PfRh5 forms a complex with cysteine-rich protective antigen (CyRPA) and P. falciparum Rh5 interacting protein (PfRipr). The PfRh5/CyRPA/PfRipr complex plays an essential role for invasion of P. falciparum into human erythrocytes through binding the receptor basigin. CyRPA displays a canonical six-bladed β-propeller fold, and the inhibitory monoclonal is shown to block formation of the PfRh5/CyRPA complex. Within the β-propeller structure are four intra-sheet disulfide bonds (Cys19-Cys35, Cys90-Cys92, Cys151-Cys169 and Cys229-Cys239) and one inter-sheet disulfide bond (Cys274-Cys298).

To provide a structural basis for understanding the function of this complex and its components we have determined the structure of CyRPA in its free form. Crystals were also obtained of uncomplexed CyRPA; this structure was determined by molecular replacement, using the CyRPA component of the Fab-complexed structure as a search model, and subsequently refined using diffraction data to 3.09 Å resolution. The crystal of uncomplexed CyRPA contains four copies of the protein in the crystallographic asymmetric unit, arranged with approximate 222-point group symmetry. Within this tetramer, a pairwise association of CyRPA molecules is mediated by the formation of two eight-strand anti-parallel β-sheets, one (termed sheet ‘6–6’) comprises two copies of the sixth β-sheet of the CyRPA monomer and the second (termed sheet ‘5–5’) comprises two copies of the (adjacent) fifth β-sheet of the CyRPA monomer. In each case, formation of the eight-stranded sheet is mediated by the respective outermost strands of the two constituent four-stranded sheets. These dimers of CyRPA monomers then associate with each other via the formation of a β-sandwich comprising sheet 6–6 of one CyRPA dimer and sheet 6–6 of the second CyRPA dimer. The monomer-monomer interfaces, although extensive, are most likely an artefact of crystallization, as we find no evidence for higher-order association upon SEC of CyRPA. However, we cannot rule out such associations occurring within the hetero-complexes formed by CyRPA and its partner proteins on the surface of the merozoite. The closest structural homologue to CyRPA is the attachment glycoprotein of a henipah virus which binds to ephrinB2 and is important for host cell entry; however, it also has some similarity to bacterial and viral sialidases all of which have a six-bladed β-propeller fold. CyRPA lacks some of the important amino acid motifs required for it to be an active sialidase, and the recombinant form of the protein did not have sialidase activity suggesting it is only distantly related to these enzymes.

>[4x]GTSRHVFIRTELSFIKNNVPCIRDMFFIYKRELYNICLDDLKGEEDETHIYVQKKVKDSWITLNDLFKETDLTGRPHIFAYVDVEEIIILLCEDEEFSNRKKDMTCHRFYSNDGKEYNNAEITISDYILKDKLLSSYVSLPLKIENREYFLICGVSPYKFKDDNKKDDILCMASHDKGETWGTKIVIKYDNYKLGVQYFFLRPYISKNDLSFHFYVGDNINNVKNVNFIECTHEKDLEFVCSNRDFLKDNKVLQDVSTLNDEYIVSYGNDNNFAECYIFFNNENSILIKPEKYGNTAAGCYGGTFVKIDENRALFIYSSSQGIYNIHTIYYANYE> AIGPVADLTISNGAVSPDGFSRQAILVNDVFPSPLITGNKGDRFQLNVIDNMTNHTMLKSTSIHWHGFFQHGTNWADGPAFVNQCPISTGHAFLYDFQVPDQAGTFWYHSHLSTQYCDGLRGPIVVYDPNDPHASLYDVDDDSTVITLADWYHLAAKVGAPVPTADATLINGLGRSAATLAADLAVITVTKGKRY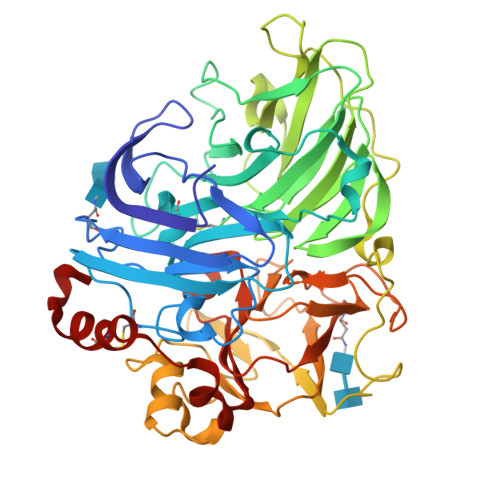RFRLVSLSCDPNYTFSIDGHSLTVIEADSVNLKPHTVDSLQIFAAQRYSFVLNADQDVDNYWIRALPNSGTQNFAGGTNSAILRYDGAAPVEPTTSQTPSTNPLVESALTTLKGTAAPGSPTPGGVDLALNMAFGFAGGNFTINGASFTPPTVPVLLQILSGAQSAADLLPAGSVYSLPANADIEISLPATAAAPGFPHPFHLHGHVFAVVRSAGSSTYNYANPVYRDVVSTGAPGDNVTIRFRTDNPGPWFLHCHIDFHLEAGFAVVMAEDIPDVAATNPVPQAWSDLCPTYDALSPDDQX Fenoterol | C17 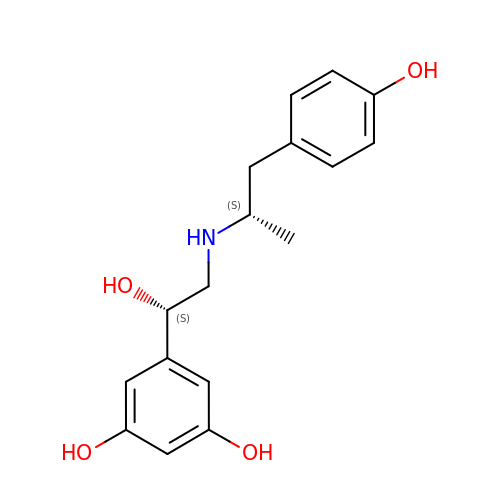H21 N O4 | LSLYOANBFKQKPT-APPDUMDISA-N>HHHHHHMSAIKPDMKINLRMEGNVNGHHFVIDGDGTGKPFEGKQSMDLEVKEGGPLPFAFDILTTAFHYGNRVFAEYPDHIQDYFKQSFPKGYSWERSLTFEDGGICIARNDITMEGDTFYNKVRFHGVNFPANGP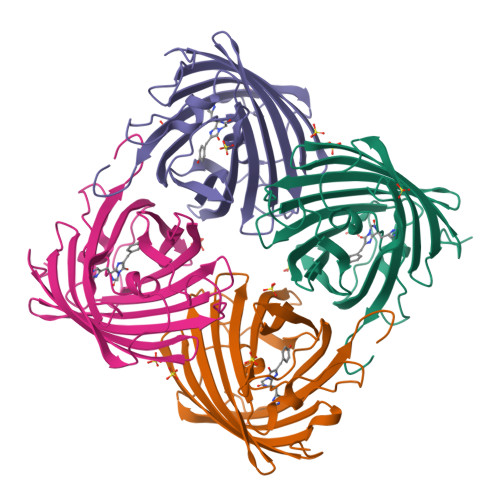VMQKKTLKWEPSTEKMYVRDGVLTGDITMALLLEGNAHYRCDSRTTYKAKEKGVKLPGYHLVDHCIEILSHDKDYNKVKLYEHAVAHSGLPDN[4x]9-AMINO-N-[2-(4-MORPHOLINYL)ETHYL]-4-ACRIDINECARBOXAMIDE 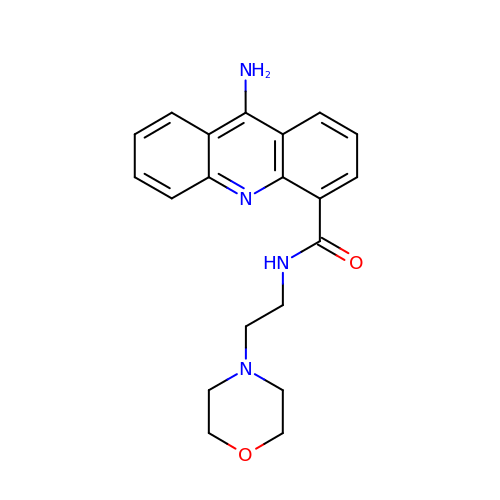| C20 H22 N4 O2 | CUJXCTHCYRNLIF-UHFFFAOYSA-N>MGNDISLIALLAFSTLLPFIIASGTCFVKFSIVFVMVRNALGLQQIPSNMTLNGVALLLSMFVMWPIMHDAYVYFEDEDVTFNDISSLSKHVDEGLDGYRDYLIKYSDRELVQFFENAQLKRQYGEETETVKRDKDEIEKPSIFALLPAYALSEIKSAFKIGFYLYLPFVVVDLVVSSVLLALGMMMMSPVTISTPIKLVLFVALDGWTLLSKGLILQYMDIAT[5x];> MFYALYFEIHHLVASAALGFARVAPIFFFLPFLNSGVLSGAPRNAIIILVALGVWPHALNEAPPFLSVAMIPLVLQEAAVGVMLGCLLSWPFWVMHALGCIIDNQRGATLSSSIDPANGIDTSEMANFLNMFAAVVYLQNGGLVTMVDVLNKSYQLCDPMNECTPSLPPLLTFINQVAQNALVLASPVVLVLLLSEVFLGLLSRFAPQMNAFAISLTVKSGIAVLIMLLYFSPVLPDNVLRLSFQATGLSSWFYERGATHVLE;>MDDLVFAGNKALYLVLILSGWPTIVATIIGLLVGLFQTVTQLQEQTLPFGIKLLGVCLCLFLLSGWYGEVLLSYGRQVIFLALAKG[4x];>MSIATIVPENAVIGQAVNIRSMETDIVSLDDRLLQAFSGSAIATAVDKQTITNRIEDPNLVTDPKELAISQEMISDYNLYVSMVSTLTRKGVGAVETLLRS[6x];>[72x]MATPWSGYLDDVSAKFDTGVDNLQTQVTEALDKLAAKPSDPALLAAYQSKLSEYNLYRNAQSNTVKVFKDIDAAIIQNFR;>MKTHILLARVLACAALVLVTPGYSSEKIPVTGSGFVAKDDSLRTFFDAMALQLKEPVIVSKMAARKKITGNFEFHDPNALLEKLSLQLGLIWYFDGQAIYIYDASEMRNAVVSLRNVSLNEFNNFLKRSGLYNKNYPLRGDNRKGTFYVSGPPVYVDMVVNAATMMDKQNDGIELGRQKIGVMRLNNTFVGDRTYNLRDQKMVIPGIATAIERLLQGEEQPLGNIVSSEPPAMPAFSANGEKGKAANYAGGMSLQEALKQNAAAGNIKIVAYPDTNSLLVKGTAEQVHFIEMLVKALDVAKRHVELSLWIVDLNKSDLERLGTSWSGSITIGDKLGVSLNQSSISTLDGSRFIAAVNALEEKKQATVVSRPVLLTQENVPAIFDNNRTFYTKLIGERNVALEHVTYGTMIRVLPRFSADGQIEMSLDIEDGNDKTPQSDTTTSVDALPEVGRTLISTIARVPHGKSLLVGGYTRDANTDTVQSIPFLGKLPLIGSLFRYSSKNKSNVVRVFMIEPKEIVDPLTPDASESVNNILKQSGAWSGDDKLQKWVRVYLDRGQEAIK[16x];>[24x]MIRRYLYTFLLVMTLAGCKDKDLLKGLDQEQANEVIAVLQMHNIEANKIDSGKLGYSITVAEPDFTAAVYWIKTYQLPPRPRVEIAQMFPADSLVSSPRAEKARLYSAIEQRLEQSLQTMEGVLSARVHISYDIDAGENGRPPKPVHLSALAVYERGSPLAHQISDIKRFLKNSFADVDYDNISVVLSERSDAQLQAPGTPVKRNSFATSWIVLIILLSVMSAGFGVWYYKNHYARNKKGITADDKAK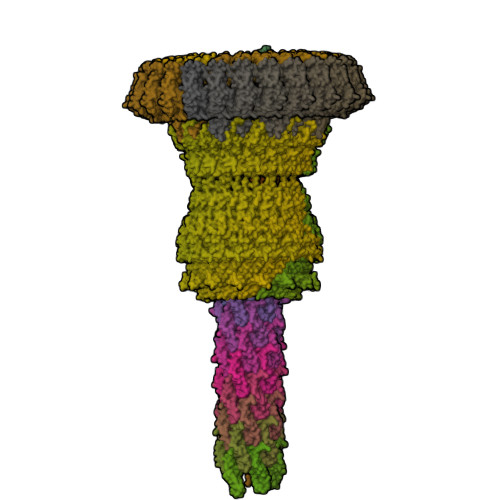SSNE;>METSKEKTITSPGPYIVRLLNSSLNGCEFPLLTGRTLFVVGQSDALTASGQLPDIPADSFFIPLDHGGVNFEIQVDTDATEIILHELKEGNSESRSVQLNTPIQVGELLILIRPESEPWVPEQPEKLETSAKKNEPRFKNGIVAALAGFFILGIGTVGTLWILNSPQRQAAELDSLLGQEKERFQVLPGRDKMLYVAAQNERDTLWARQVLARGDYDKNARVINENEENKRISIWLDTYYPQLAYYRIHFDEPRKPVFWLSRQRNTMSKKELEVLSQKLRALMPYADSVNITLMDDVTAAGQAEAGLKQQALPYSRRNHKGGVTFVIQGALDDVEILRARQFVDSYYRTWGGRYVQFAIELKDDWLKGRSFQYGAEGYIKMSPGHWYFPSPL[24x]> MSMTILPLELIDKCIGSNLWVIMKSEREFAGTLVGFDDYVN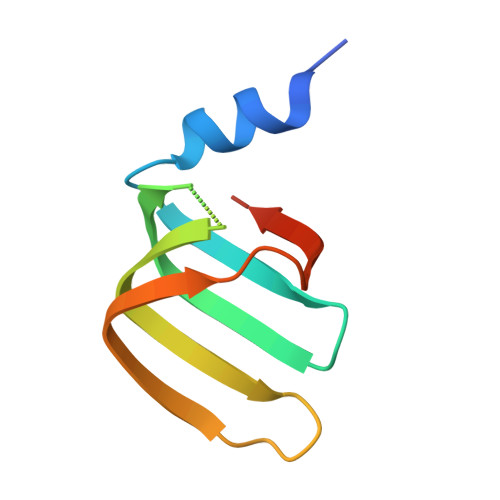IVLKDVTEYDTVTGVTEKHSEMLLNGNGMCMLIPGGKPE>MSLGMHLPGGIVENVRKRPGMYCGDVGEYGLHHLVYFLLDVAYEEARRGECRDVVLEVGGDGSIALFCTSRTVTAENLVRVATGAGFLGRPPGDGWGWDSMLVVSLALSSRYQVDIWADGRQWRVMGEHGHPQGEGAAVTPMEPMPVSAERGVRVHFVPDATIFEVLAFDRARLSRRCNELAALAPGLRVSFADLQRGERTLWHLPGGVAQWAHVLTEARPQLHPEPVVFDFTWDGLRVQCALQWCEDEDSTLLSFANAV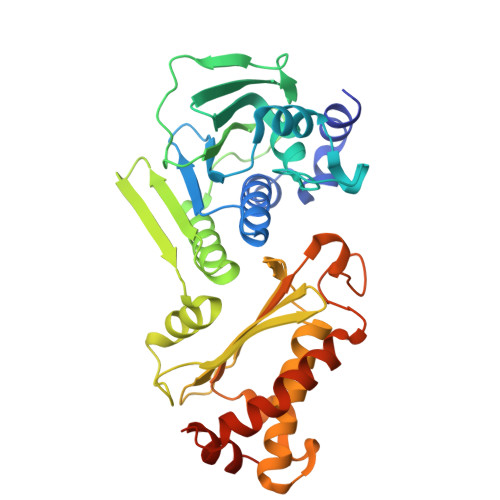RTVRHGAHVKGVTQALRGALAKLSGETRGAFPWARVAQGLTAIVAVSGPRRQMAFAGPTKELLAIPGLEEAIRKQLQPLFIELLREHPVTPALLARRTSGSEGHHHHHH[2x]> GPGSEFEKPPKRKIVLLMAYSGKGYHGMQRNVGSSQFKTIEDDLVSALVRSGCIPENHGEDMRKMSFQRCARTDKGVSAAGQVVSLKVWLIDDILEKINSHLPSHIRILGLKRVTGGFNSKNRCDARTYCYLLPTFAFAHKDRDVQDETYRLSAETLQQVNRLLACYKGTHNFHNFTSQKGPQDPSACRYILEMYCEEPFVREGLEFAVIRVKGQSFMMHQIRKMVGLVVAIVKGYAPESVLERSWGTEKVDVPKAPGLGLVLERVHFEKYNQRFGNDGLHEPLDW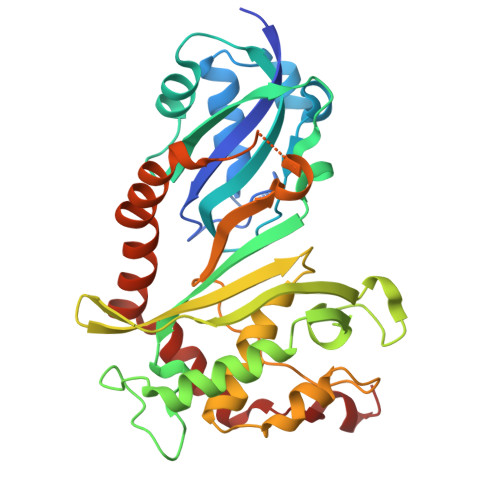AQEEGKVAAFKEEHIYPTIIGTERDERSMAQWLSTLPIHNFSATALTAGG> TTTVGLVCKDGVVMATEKRATMGNFIASKAAKKIYQIADRMAMTTAGSVGDAQFLARIIKIEANLYEIRRERKPTVRAIATLTSNLLNSYRYFPYLVQLLIGGIDSEGKSIYSIDPIGGAIEEKDIVATGSGSLTAYGVLEDRFTPEIGVDEAVELAVRAIYSAMKRDSASGDGIDVVKITEDEFYQYSPEEVEQILAKFR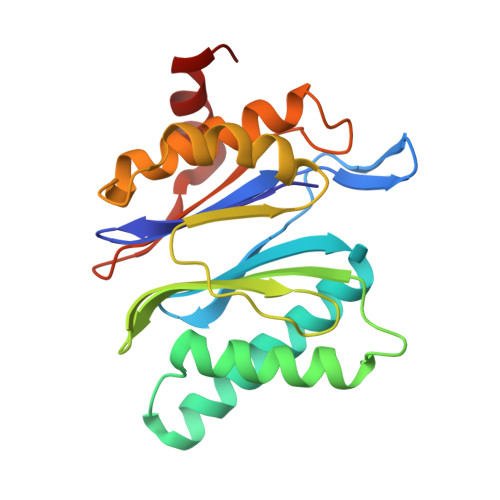K> ASPDDNFSPETLQFLRNNTGLDGEQWNNIMKLINKPQQDDLNWIKYYGYCEDIEDERGYTIGLFGATTGGSRDTHPDGPDLFK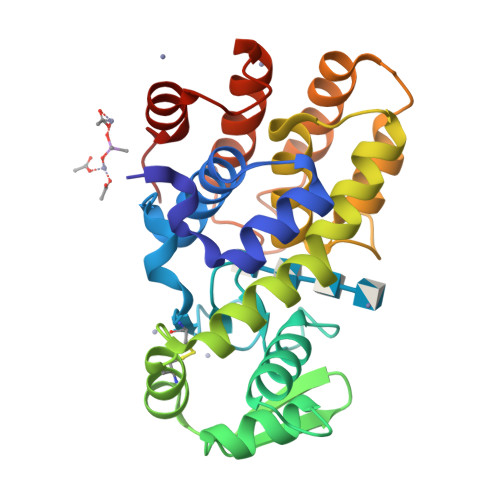AYDAAKGASNPSADGALKRLGINGKMKGSILEIKDSEKVFCGKIKKLQNDAAWRKAMWETFYNVYIRYSVEQARQRGFTSAVTIGSFVDTALNQGATGGSDTLQGLLARSGSSSNEKTFMKNFHAKRTLVVDTNKYNKPPNGKNRVKQWDTLVDMGKMNLKNVDSEIAQVTDWEMK>XGQLEEIAKQLEEIAWQLEEIAQGX[4x];>XGQLKKIAKQLKKIAYQL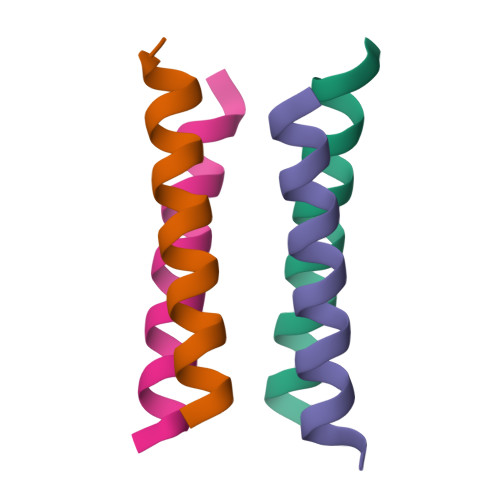KKIAQGX[4x]(1R,2Z,3R,5E,7E,9beta,17beta)-2-(2-hydroxyethylidene)-17-[(2R)-6-hydroxy-6-methylheptan-2-yl]-9-(prop-2-en-1-yl)-9,10-secoestra-5,7-diene-1,3-diol | C31 H50 O4 | 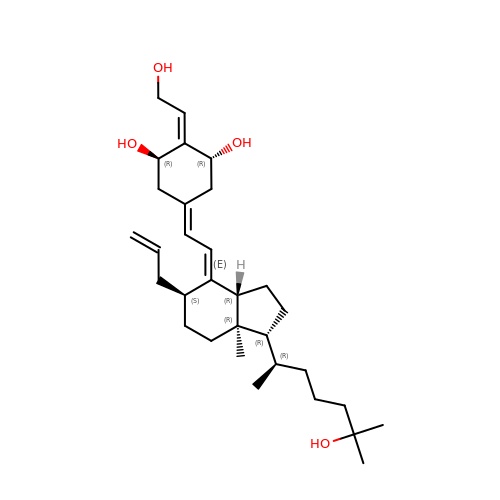VQPYCEUJPLIUFQ-ZVOFGSMJSA-N> VHWTQEERDEISKTFQGTDMKTVVTQALDRMFKVYPWTNRYFQKRTDFRSSIHAGIVVGALQDAVKHMDD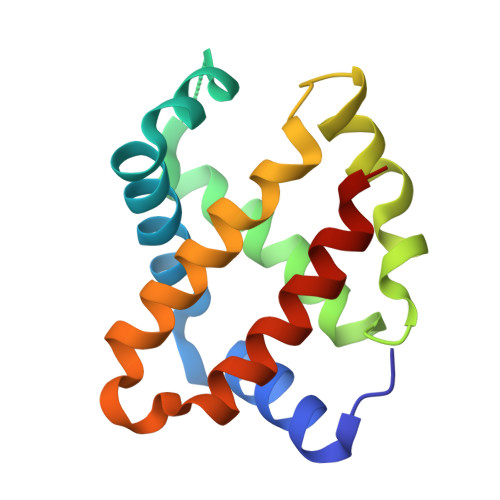VKTLFKDLSKKHADDLHVDPGSFHLLTDCIIVELAYLRKDCFTPHIQGIWDKFFEVVIDAISKQY>SATNGKLFPWAQIRLPTAVVPLRYELSLHPNLTSMTFRGSVTISVQALQVTWNIILHSTGHNISRVTFMSAVSSQEKQAEILEYAYHGQIAIVAPEALLAGHNYTLKIEYSANISSSYYGFYGFSYTDESNEKKYFAATQFEPLAARSAFPCFDEPAFKATFIIKIIRDEQYTALSNMPKKSSVVLDDGLVQDEFSESVKMSTYLVAFIVGEMKNLSQDVNGTLVSIYAVPEKIGQVHYALETTVKLLEFFQNYFEIQYPLKKLDLVAIPDFEAGAMENWGLLTFREETLLYDSNTSSMADRKLVTKIIAHELAHQWFGNLVTMKWWNDLWLNEGFATFMEYFSLEKIFKELSSYEDFLDARFKTMKKDSLNSSHPISSSVQSSEQIEEMFDSLSYFKGSSLLLMLKTYLSEDVFQHAVVLYLHNHSYASIQSDDLWDSFNEVTNQTLDVKRMMKTWTLQKGFPLVTVQKKGKELFIQQERFFLNMKPEIQPSDTSYLWHIPLSYVTEGRNYSKYQSVSLLDKKSGVINLTEEVLWVKVNINMNGYYIVHYADDDWEALIHQLKINPYVLSDKDRANLINNIFELAGLGKVPLKRAFDLINYLGNENHTAPITEALFQTDLIYNLLEKLGYMDLASRLVTRVFKLLQNQIQQQTWTDEGTPSMRELRSALLEFACTHNLGNCSTTAMKLFDDWMASNGTQSLPTDVMTTVFKVGAKTDKGWSFLLGKYISIGSEAEKNKILEALASSEDVRKLYWLMKSSLNGDNFRTQKLSFIIRTVGRHFPGHLLAWDFVKENWNKLVQKFPLGSYTIQNIVAGSTYLFSTKTHLSEVQAFFENQSEATFRLRCVQEALEVIQLNIQWMEKNLKSLTWWL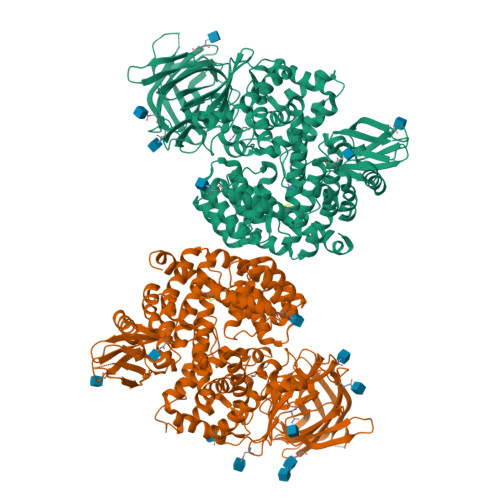[2x]> MQFTLAAAAALFGASALAAPASPGSTGAPPDPNMYENIDIADFNVRKGEDGTIKYVNFKLSGDDADGLLCE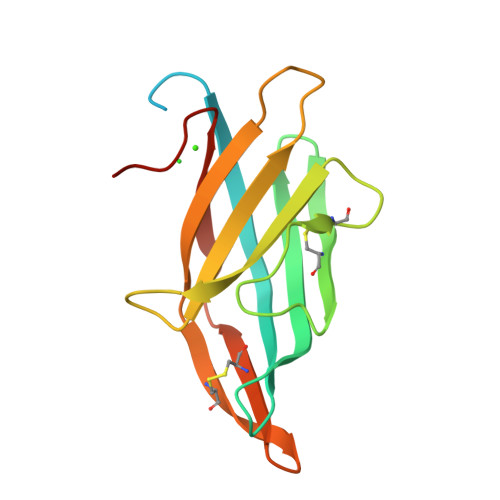AQNPGLPSNVITCGESKYRFALSSGKQYEFALSLYHELGLAVGFYGTGEIFTHCRAGGLGDFICQQQNPTTIVIDSLPDAPAEA>MTPSRPSPDFPDGGFVQVRGARQHNLKDISVKVPRDALVVFTGVSGSGKSSLAFGTLYAEAQRRYLESVSPYARRLFNQAGVPDVDAIDGLPPAVALQQARGTPTARSSVGSVTTLSNLLRMLYSRAGDYPPGQGIVYAEGFSPNTPEGACPECHGLGRVYTVTEDSMVPDPSLTIRERAVAAWPQAWGGQNQRDILVTLGIDVDVPWRELPEETRHWILFTDEQPVVPVYPGLTPAETQRALKKKMEPSYMGTFSSARRHVLHTFANTESASMKKRVQGYMISEECPLCHGKRLRQEALNVTFAGLDITELSRLPLARVSELLRPYAEEREPGHAERVKNRPEQAIALQRMAADLVKRLDVLLHLGLGYLGLDRSTPTLSPGELQRLRLATQLYSNLFGVVYVLDEPSAGLHPADTEALLSALENLKRGGNSLFVVEHDLDVIRRADWLVDVGPEAGEKGGEILYSGPPEGLKHVPESQTGQYLFADRHTEPHTPREPAGWLELNGVTRNNLDNLDVRFPLGVMTSVTGVSGSGKSTLVSQALVDALAAHFGQPVNPDPEDDEDPADHTAGSARLGGDLAQITRLVRVDQKPIGRTPRSNMATYTGLFDQVRKLFAATPLAKKRGYNAGRFSFNVKGGRCEHCQGEGWVMVELLFLPSVYAPCPVCHGTRYNAETLEVEYRGKNIADVLALTVDEAHDFFADESAIFRALDTLREVGLGYLRLGQPATELSGGEAQRIKLATELRRSGRGGTVYVLDEPTTGLHPADVERLQRQLVKLVDAGNTVIAVEHKMQVVAASDWVLD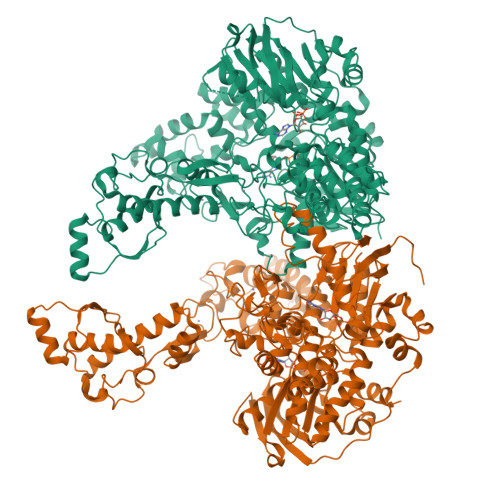IGPGAGEDGGRLVAQGTPAEVAQAAGSVTAPYLRAALR[3x]> ELTPDQQTLLHFIMDSYNKQRMPQEITNKILKEEFSAEENFLILTEMATNHVQVLV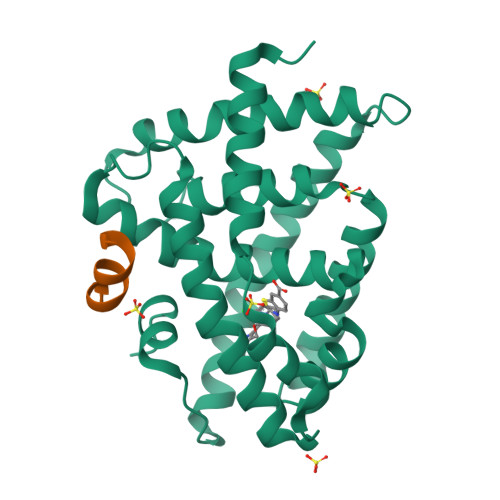EFTKKLPGFQTLDHEDQIALLKGSAVEAMFLRSAEIFNKKLPSGHSDLLEERIRNSGISDEYITPMFSFYKSIGELKMTQEEYALLTAIVILSPDRQYIKDREAVEKLQEPLLDVLQKLCKIHQPENPQHFAELLGRLTELRTFNHHHAEMLMSWRVNDHKFTPLLEEIWDVQ;> DHQLLRYLLDK>MEIRKKLVVPSKYGTKCPYTMKPKYITVHNTYNDAPAENEVNYMITNNNEVSFHVAVDDKQAIQGIPWERNAWACGDGNGPGNRESISVEICYSKSGGDRYYKAENNAVDVVRQLMSMYNIPIENVRTHQSWSGKYCP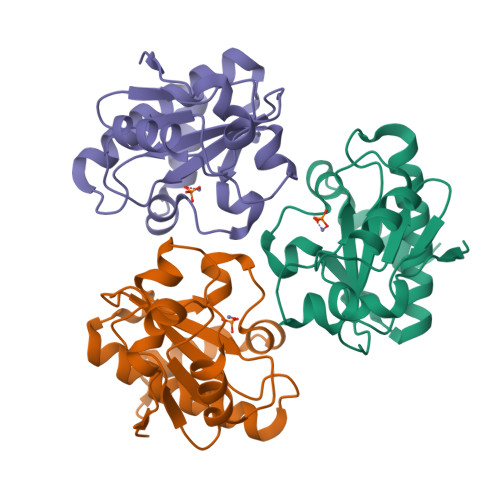HRMLAEGRWGAFIQKVKSGNV[3x]> GPMAVGPEPLVPSPQPVPEVPSLDPTVLPLYSLGPSGQLAETPAEVFQALEQLGHQAFRPGQERAVMRILSGISTLLVLPTGAGKSLCYQLPALLYSRRSPCLTLVVSPLLSLMDDQVSGLPPCLKAACIHSGMTRKQRESVLQKIRAAQVHVLMLTPEALVGAGGLPPAAQLPPVAFACIDEAHCLSQWSHNFRPCYLRVCKVLRERMGVHCFLGLTATATRRTASDVAQHLAVAEEPDLHGPAPVPTNLHLSVSMDRDTDQALLTLLQGKRFQNLDSIIIYCNRREDTERIAALLRTCLHAAWVPGSGGRAPKTTAEAYHAGMCSRERRRVQRAFMQGQLRVVVATVAFGMGLDRPDVRAVLHLGLPPSFESYVQAVGRAGRDGQPAHCHLFLQPQGEDLRELRRHVHADSTDFLAVKRLVQRVFPACTCTCTRPPSEQEGAVGGERPVPKYPPQEAEQLSHQAAPGPRRVCMGHERALPIQLTVQALDMPEEAIETLLCYLELHPHHWLELLATTYTHCRLNCPGGPAQLQALAHRCPPLAVCLAQQLPEDPGQGSSSVEFDMVKLVDSMGWELASVRRALCQLQWDHEPRTGVRRGTGVLVEFSELAFHLRSPGDLTAEEKDQICDFLYGRVQARERQALARLRRTFQAFHSVAFPSCGPCLEQQDEERSTRLKDLLGRYFEEEEGQEP

RecQ proteins are ATP- and DNA-dependent super family 2 (SF2) helicases and separate double stranded DNA (dsDNA) in a 3′ to 5′ direction. Remarkably, RecQ4 entirely lacks the RQC domain, yet its helicase activity is required for various DNA protective functions. Here we present the crystal structure of the human RecQ4 helicase, encompassing its central ATPase domain and a large fraction of its unique C-terminus. Downstream of the ATPase core, we identify a novel domain, which features homology to WH domains of various prokaryotic DNA-binding proteins and coordinates a Zn2+-ion, yet lacks structural resemblance to the conserved RQC domain.

The RecQ4427-1116 model was refined to a resolution of 2.75 Å and contains aa 449–1111. Two disordered regions within the C-terminus (aa 858–882 and aa 975–983) and two short areas within the ATPase domain (aa 664–667 and aa 727–734) are not resolved. Two ‘bridging’ α-helices (aa 823–835 and aa 1046–1079) link HD2 to a unique domain further downstream (aa 836–1045), which is not present in other RecQ helicases. Zn2+-coordination is accomplished via three cysteines and a histidine, which are located in the loop region between helix α12 and β-strand β13. The two bridging helices thus connect the HD2 to the R4ZBD in a hinge-like fashion, with the joint of the hinge being located at the HD2–bridge–helix interface. The R4ZBD, on the other side of this lever, interacts with HD1 through several salt bridges and hydrogen bonds. The R4ZBD of RecQ4 is located directly adjacent to HD1 and thus assumes a unique position among the characterized RecQ proteins, as their C-terminal extensions are located on the opposite side, directly adjacent to HD2. Our structural alignment between RecQ4 and other known RecQ structures revealed that RecQ4s bridging helix α11, the downstream part of bridging helix α19 and helix α20, together, mimic the conserved structure and exact position of the RQC-Zn2+-binding domain of other RecQ helicases, with the notable difference that RecQ4 does not coordinate a zinc ion at this position. In agreement with our ARL data, the RecQ4 structure exhibits a highly electropositive cleft between the R4ZBD and HD1, poised to bind the negatively charged ssDNA backbone. Our in vitro biochemical analysis of the RecQ4427–1116 variant provides evidence that our model features all necessary structural elements for ATP- and DNA-dependent helicase activity.>[4x]HMSVNKVTCLVCRKGDNDEFLLLCDGCDRGCHIYC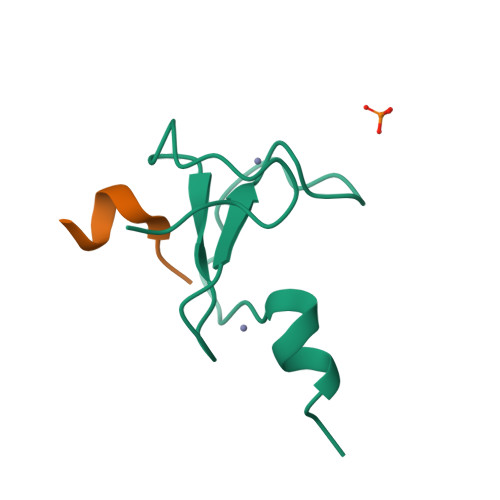HRPKMEAVPEGDWFCTVCLAQQV;>[3x]ARTAATARKS>MNDSSVIYRAIVTSKFRTEKMLNFYNSIGSGPDKNTIFITFGRSEPWSSNENEVGFAPPYPTDSVLGVTDMWTHMMGTVKVLPSMLDAVIPRRDWGDTRYPDPYTFRINDIVVCNSAPYNATESGAGWLVYRCLDVPDTGMCSIASLTDKDECLKLGGKWTPSARSMTPPEGRGDAEGTIEPGDGYVWEYLFEIPPDVSINRCTNEYIVVPWPEELKEDPTRWGYEDNLTWQQDDFGLIYRVKANTIRFKAYLDSVYFPEAALPGNKGFRQISIITNPLEAKAHPNDPNVKAEKDYYDPEDLMRHSGEMIYMENR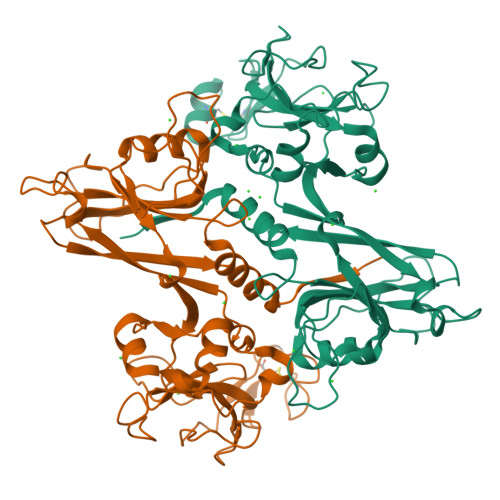PPIIMAMDQTEEINILFTF[4x]At the inner surface of fly photoreceptor rhabdomeric membranes, the master scaffold protein INAD (encoded by inaD for inactivation no after potential D and contains 5 PDZ domains arranged in tandem) forms stoichiometric multi-molecular complexes with phospholipase Cβ (NORPA), Ca2+-permeable transient receptor potential (TRP) channel and eye-specific protein kinase C (eye-PKC). In this study, we show that the PDZ45 tandem of INAD functions as a supramodule binding to the entire C-terminal coiled-coil domain and PDZ-binding motif of NORPA (CC-PBM) with an unexpectedly high affinity. Our biochemical and structural studies demonstrate that INADL PDZ89 forms a supramodule and binds to the entire C-terminal coiled-coil domain of PLCβ4 in a manner that is strikingly similar to that of the INAD–NORPA complex. The striking similarity between the PDZ scaffold and PLCβ interactions at the molecular level might point to an evolutionarily conserved molecular adaption in PLCβ signaling in the animal kingdom.

Multiple years of attempts to crystallize the complex prepared from the wildtype INAD PDZ45 and NORPA CC-PBM all failed, even though our NMR-based study indicated that the PDZ45–NORPA CC-PBM complex is conformationally homogeneous in solution. We substituted the eight Lys residues with Ala residues (designated as CC8KA-PBM) with the rationale that such substitutions should not impair the helical conformation of α2 but might create a new crystal packing surface for the PDZ45–NORPA CC-PBM complex. Satisfyingly, the NORPA CC8KA-PBM–INAD PDZ45 complex could be crystallized and the structure of the complex was solved at the resolution of 3.2 Å by molecular replacement methods, using the apo-form NORPA CC-PBM structure as the search model. The most important feature of the complex is that both PDZ domains of the PDZ45 tandem and both the coiled coil and PBM of NORPA participate cooperatively to form a highly stable INAD–NORPA complex burying an extensive interaction surface area of ~1373 Å2. PDZ45 binding stabilizes the conformation of NORPA's C-terminal 16 amino acids by extending the α4 helix for five more turns, immediately followed by a four-residue β-strand corresponding to the PBM of NORPA. Structural alignment analysis showed that the INAD PDZ45 tandem, including the inter-PDZ domain interactions, underwent minimal conformational changes upon binding to NORPA CC-PBM. The binding interface of the PDZ45–NORPA CC-PBM complex can be divided into three distinct sites: the PDZ5–PBM interaction site (site 1), the PDZ5/CC packing site (site 2), and the PDZ4/CC binding site (site 3). In site 1, NORPA PBM (‘EFYA’) inserts into the βB’/αB’ groove of PDZ5 following the typical PDZ–ligand interaction mode. In the NORPA–INAD complex, INAD PDZ45 binds to one face of the NORPA CC with the two PDZ domains crossing over the α2, α3, and α4 helices.

> AEPPLVFEPVTLESLRQEAGFQAVGAAQIAELDTLRAAHAAERTSVQKTQNAAIDKLIKGKSKDDIRNDANIKNSINDQTKQWTDMIARHRKEEWDMLRQHVQDSQDAMKALMLTVQAAQIKQLEDRHARDIKDLNAKQAKMSADTAKEVQNDKTLKTKNEKDRRLREKRQNNVKRFMEEKKQIGVKQGRAMEKLKLAHSKQIEEFSTDVQKLMDMYKIEEEAYKTQGKTEFYA;> ATAEIKPNKKILIELKVEKKPMGVIVCGGKNNHVTTGCVITHVYPEGQVAADKRLKIFDHICDINGTPIHVGSMTTLKVHQLFHTTYEKAVTLTVFRADPPELEKFNVDLMKKAGKELGLSLSPNEIGCTIADLIQGQYPEIDSKLQRGDIITKFNGDALEGLPFQVCYALFKGANGKVSMEVTRPKPTLRTEA Multi-subunit SMC complexes control chromosome superstructure and promote chromosome disjunction, conceivably by actively translocating along DNA double helices. SMC subunits comprise an ABC ATPase “head” and a “hinge” dimerization domain connected by a 49 nm coiled-coil “arm. The heads undergo ATP-dependent engagement and disengagement to drive SMC action on the chromosome. Here, we elucidate the architecture of prokaryotic Smc dimers by high-throughput cysteine cross-linking and crystallography.

To better define the structural differences between Smc heads aligned at the end of the Smc rod and those engaged via ATP, we solved another crystal structure: “BsSmcHd-CC30:ATPγS-ScpAC” comprising ATPγS bound Bs Smc(E1118Q) heads with 30-residue coiled coils associated with the C-terminal winged-helix domain of Bs ScpA (ScpAC). The arrangement of the two head domains in BsSmcHd-CC30:ATPγS-ScpAC shows a high degree of similarity (RMSD < 1 Å) with a previously solved structure of an ATP dimer of Pf Smc heads lacking coiled coils and ScpA (Lammens et al., 2004). We measured the Cα-Cα distances for S152-S152′ (located on the Smc head) and D193-D193′ (located at the head-proximal coiled coil) on the BsSmcHd-CC30 dimer at 21.7 and 77.0 Å, respectively. These large distances are incompatible with their efficient cross-linking by BMOE, implying that cysteine cross-linking takes place on Smc dimers with disengaged heads. To convert the rod-shaped into the ATP-engaged state, we need two operations: the sliding of Smc heads toward each other along an axis connecting the two ATP-binding pockets by about 10 Å and the tilting of one Smc head relative to the other head by about 85° around a similar axis. Both transformations bring about the dissolution of the Smc rod by positioning the head-proximal Smc coiled coils at a distance.

>[2x]MFLKRLDVIGFKSFAERISVDFVKGVTAVVGPNGSGKSNITDAIRWVLGEQSARSLRGGKMEDIIFAGSDSRKRLNLAEVTLTLDNDDHFLPIDFHEVSVTRRVYRSGESEFLINNQPCRLKDIIDLFMDSGLGKEAFSIISQGKVEEILSSKAEDRRSIFEEAAGVLKYKTRKKKAENKLFETQDNLNRVEDILHELEGQVEPLKIQASIAKDYLEKKSGGSLIKLAIEELGTVNLGSIDEFERVNERYKFLSEQKEDLTEAKNTLFQVIEEMDEEMTKRFNDTFVQIRSHFDQVFRSLFGGGRAELRLTDPNDLLHSGVEIIAQPPGKKLQNLNLLSGGERALTAIALLFSILKVRPVPFCVLDQVEAALDEANVFRFAQYLKKYSSDTQFIVITHRKGTMEEADVLYGVTMQESGVSKVISVKLEETKEFVQ;>NRPMETTITRQDIPIEARMNEIVHSLKSRGTRINFMDLFPYEQKEHLVVTFLAVLELMKNQLVLIEQEHNFSDIYITGSESIHGAVDKL[2x]Sandercyanin (SFP) is a BV-binding lipocalin protein found in the skin mucus of the Canadian walleye, Stizostedion vitreum (formerly Sander vitreus). BV associates non-covalently to each SFP monomer in a ZZZssa conformation and is stabilized by aromatic stacking, hydrophobic interactions, and water-mediated H-bonding inside the lipocalin-like beta-barrel fold of SFP. The binding of BV induces tetramerization of SFP via interaction between amino acid residues from adjacent monomeric subunits. Using a combination of designed site-directed mutations, X-ray crystallography, UV/VIS, and resonance Raman spectroscopy, we have identified multiple conformations of BV that are stabilized in the binding pocket of SFP.

Two mutations – L135E (from interface 1) and V71E (from interface 2) stayed monomers on binding to BV as identified by size-exclusion chromatography profiles. Mutating these hydrophobic residues into polar/charged residues disrupted the binding interface. The purified L135E and V71E variants of SFP (the BV-bound monomeric variants) showed a distinct blue-green coloration (ESI Fig. S1†) under physiological conditions, unlike wild-type protein that appears deep-blue in color. The absorbance spectra of BV-bound V71E and L135E show maxima at 380 nm and an attenuated red-shifted broad peak at the far-red wavelengths (∼680–700 nm) compared to the wild-type protein, where the red-absorbance is at 630 nm. The V71E and L135E mutations showed an order of magnitude reduction, with fluorescence quantum yields of 0.003 and 0.0025, respectively (for excitation at 630 nm). Loss of oligomerization created a vacant space in the monomer near the open/wider end of the barrel, exposing BV to an aqueous environment at the site of dimerization. In the BV-binding pocket, both monomeric variants revealed a rotated D-ring pyrrole of BV around the C14–C15 single bond. Measured torsion angles were 122° and 125° (counter-clockwise) for V71E and L135E, respectively. The conformation of BV is ZZZsss in the variants compared to ZZZssa in wild-type SFP. However, in the monomeric forms, the orientation of the D-ring of BV is stabilized by interactions with the A-ring of BV (the D-ring moves closer to the A-ring of BV) and stacking interactions with the Y142 side chain (which rotates to stack with the D-ring). In the V71E structure, water molecules occupy the original space vacated by the reoriented side-chains of F55 and Y142.

> MFIKPGRCPKPAVQEDFDAARYLGVWYDIQRLPNKFQKGECATATYSLSPGEGFSVFNRERLANGTIKSVIGSAIAEDPCEPAKLQFFHENAAPVPYWVLSTDYDNYALVYSCINLGASHAAYASIVSRQPTLPEETIKKLQGTMSSFGVGVDTLLTTNQDAAYCSAMNQKLAAALEHHHHHH Here we report the identification, purification and characterization of a novel anticoagulant ringhalexin (Ringhals extrinsic tenase complex inhibitor) from the venom of H. haemachatus. Ringhalexin exhibited a mixed-type inhibition to FX activation by the extrinsic tenase complex and also exhibited a weak, irreversible, neurotoxicity on chick biventer cervicis muscle (CBCM) preparations. Ringhalexin, like other 3FTxs, has three β-stranded loops extending from a central core containing four conserved disulfide bonds which resembles the three outstretched fingers of a hand. Thus, ringhalexin exhibits mixed-type inhibition of FX activation by extrinsic tenase complex.

There were three protein molecules in an asymmetric unit with each molecule consisting of residues from Arg1 to Ala65. All the three monomers are well defined in the electron density map. The model was refined to a final R value of 0.22 (Rfree = 0.27). Each monomer of the asymmetric unit consists of 6 anti-parallel β-strands (β2↓β1↑β4↓β3↑β6↓β5↑) that form two β-sheets. The first β-sheet consists of two anti-parallel β-strands, β1 (Leu2-Tyr7) and β2 (Ser11-Ile16), while the second contains four anti-parallel strands, β3 (Tyr23-Pro29), β4 (Ile39-Ala43), β5 (Cys46-Ala51) and β6 (Val53-Cys58). The fold of ringhalexin is maintained by four disulfide bonds, and these cysteines are strictly conserved among the 3FTxs. The three fingers of ringhalexin consist of the secondary structures β1Ωβ2, β3Ωβ4 and β5Ωβ6. The electrostatic surface representation shows that the molecule is predominantly positively charged with few negative patches in the surface. As shown in the case of other 3FTxs, the loop II of ringhalexin was very flexible and some of the residues showed very high B values. This flexibility suggests the possible role of loop II residues in the function of ringhalexin.

>[3x]RLCLSDYSIFSETIEICPEGHNYCFKKFPKGITRLPWVIRGCAATCPKPEAQVYVDCCARDKCNR> MADVAGTSNRDFRGREQRLFNSEQYNYNSSLNGEVSVWVYAYYSDGSVLVINKNSQYKVGISETFKVLKEGSGAKPRAIQIIFSPSVNVRTIKMAKGNAVSVPDEYLQRSHPWEATGIKYRKIKRDGEIVGYSHYFELPHEYNSISLAVSGVHKNPSSYNVGSAHNVMDVFQSCDLALRFCNRYWAELELVNHYISPNAYPYLDINNHSYGVALSNRQ

Cypoviruses, members of the family Reoviridae, subfamily Spinareovirus, possess a single capsid layer with turrets and are commonly embedded in crystalline occlusion bodies called polyhedra, which are formed in the cell cytoplasm and mainly composed of a single virus-encoded protein, polyhedrin. To ensure the delivery of virus particles to the target intestinal cells, allowing the transmission of packages of infectious virus between hosts by oral-faecal routes, polyhedra are disrupted only when they are exposed to the very alkaline pH environment found in insect midguts. The fold of all the polyhedrins is highly similar – a β-barrel core sitting on a base domain, surrounded by a common array of five helices (H1–H5). The strongest intermolecular interactions define a trimer composed of a cluster of three β-barrels sandwiched by helices top and bottom.

Base domain deletion mutants of CPV1 (CPV1Δ) and CPV4 (CPV4Δ) were produced by three steps of PCR using primers encoding a Gly-Ser-Gly linker (described in). To test this, polyhedrin proteins were made with the base domain removed by deleting residues 74–110 of CPV4 and 71–103 of CPV1 and replacing them with a flexible Gly-Ser-Gly linker (resulting in CPV4Δ and CPV1Δ respectively). Compared to wild-type CPV1, CPV1Δ crystals also had a slightly enlarged unit cell (103.9 vs. 103.0 Å). The absence of the base domain did not influence the overall structure of the trimeric building block but increased flexibility such that the electron density for 40–50 residues in the inter-trimer contact areas could not be observed. These disordered regions include the areas in CPV1 which had been shown previously to bind NTPs, so that NTPs are absent from CPV1Δ. The base domain is therefore a region that is neither required for proper folding of the protein, nor for crystal assembly, but fine-tunes the crystal, ‘locking-down’ the structure, often in conjunction with NTPs. In contrast in the base domain deletion mutants all major cavities are connected, resulting in contiguous solvent channels running through the crystal lattice. The deletion mutants are much more sensitive to alkaline buffers, even those such as glycine and borate which do not disrupt crystals of full-length polyhedrin, although CAPS could not dissolve any of the samples effectively. We also find that the whole base domain is dispensable for polyhedra formation, although the biochemical features are altered dramatically when it is removed.> GSSTNYGTIKWIFHALVFSYISFALISDKRYQKKEPLISSVHTKVKGIAEVKAEILENGMKKMVSGVFDTADYTFPLQGNSFFVMTNFIKTEGQQQGLCPDFPTART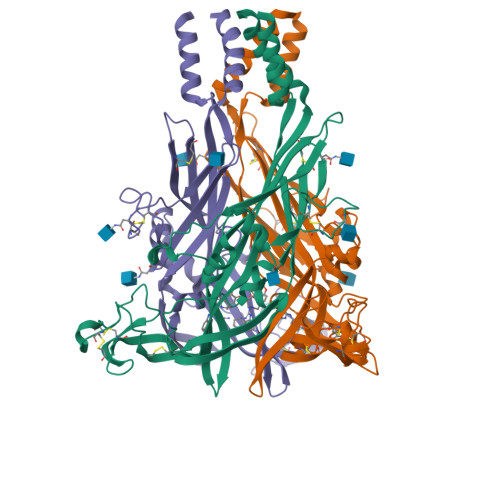ICSSDRGCKKGRMDPQSKGIQTGRCVVYKERLKTCEVSAWCPIEEVKDAPRPALLNSAENFTVLIKNNIDFPGHNYTTRNILPGVNITCTFHKTQNPQCPIFRLGDIFQETGDSFSDVAIQGGIMGIEIYWDCNLDGWFHHCRPKYSFRRLDDKTTSESLYPGYNFRYAKYYKENNVEKRTLIKVFGIRFDILVFGTGGKFNVIQLAVYIGSVISYFGLATVFIDILINTYSASS> PISPIETVPVKLKPGMDGPKVKQWPLTEEKIKALVEICTEMEKEGKISKIGPENPYNTPVFAIKKKDSTKWRKLVDFRELNKRTQDFWEVQLGIPHPAGLKKKKSVTVLDVGDAYFSVPLDEDFRKYTAFTIPSINNETPGIRYQYNVLPQGWKGSPAIFQSSMTKILEPFKKQNPDIVIYQYMDDLYVGSDLEIGQHRTKIEELRQHLLRWGLTTPDKKHQKEPPFLWMGYELHPDKWTVQPIVLPEKDSWTVNDIQKLVGKLNWASQIYPGIKVRQLSKLLRGTKALTEVIPLTEEAELELAENREILKEPVHGVYYDPSKDLIAEIQKQGQGQWTYQIYQEPFKNLKTGKYARMRGAHTNDVKQLTEAVQKITTESIVIWGKTPKFKLPIQKETWETWWTEYWQATWIPEWEFVNTPPLVKLWYQLEKEPIVGAETFYVDGAANRETKLGKAGYVTNKGRQKVVP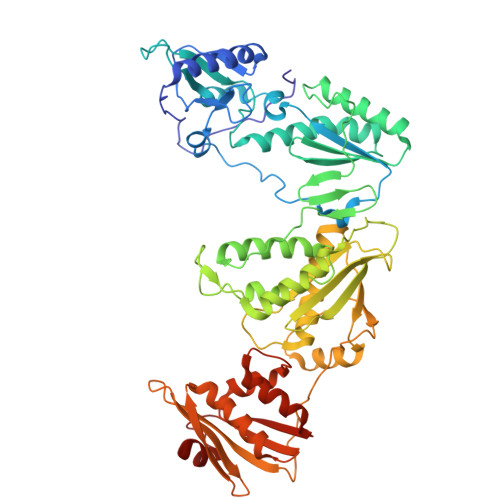LTNTTNQKTELQAIYLALQDSGLEVNIVTDSQYALGIIQAQPDKSESELVNQIIEQLIKKEKVYLAWVPAHKGIGGNEQVDKLVSAGIRKIL> MDKINLVCGSLLHNIGKIIYRGTSERAKHSKLGGDFIKSFEQFRNTELTDCIRYHHAQEITSVKSNKEKNSLFYITYIADNISSGMDRRKDLEEGAEGFNWDKKVALGSVFNVLNEKEKGRQNYSYPFVARTRIKEEPLNFPTATQNQYTTSYYDGLITDMKTILQRLKPDKEHINSLLQMMESLWSYVPSSTDKNQLVDISLYDHSRTTAAIASAIYDYFQAENITDYQKELFDYNATEFYDKNAFLMMNFDMSGVQNFIYNISGSKALKSLRARSFYLDMLLEYISDNLLEKLELSRANILYVGGGHAYLLLANTNKTKAILSDFEHDLKTWFLDKFKIDLYVAMAYTEVSANDLMNHNGHYRDIYRRLSQKTSAKKANRYTAEEILNLNHQGTENARECRECKRSDLLIEEDDICEICDSLQKVSRDLTRENIFVIANEGVLDMPFGKKMSALSYSQADKLKKSNAEVQIYAKNISEIGQNLMTRIDMGDYTYRSDFHEMLEEVEVGINRLGVLRADVDNLGQAFINGIPDDYLSISRTATFSRAMSRFFKNYLNQLLAEKSYKINVIYAGGDDLFMIGAWQDILDFSIVLKQKFADFTQNKLSISAGIGMFREKYPVARMASLTGDLEDAAKDYKPDERAVQATKNAVTLFDATNVFSWDTLENDIFVKLDAITKNFEKLDETGKAFIYRLIDLLRGVNENQQINIARLAYTLSRMEEKIGKTFAQELYNWANADRKTLIMALEIYILKTRE;> MKIIKLYFESPVHFGEKRLSESKITFSADTLFSALMIEAVGLGKEDEFYQLASNNLVKFSDAFPFIDQYYYIPKPMFNLKLEKEDENPSKAFKKLLYVPIDSLEDYLSGGLDAYFERESFNLGKLALSEKVQQHDFKDSEPYNVGTFTFKENTGLYVLIEQTHPLLEELLENLQYSGIGGKRNSGYGKFKFEILEDSDIEDLFSAKGNRKILLSGALPKDAELEQALKNASYLLERRGGFVQSDTYATNLVKKQDLYVFKSGSTFENSFDGDIYQVGKKGNHPVYKYAKSFFLEVS;>[4x]MKLVIEGTIVLKTGMHIGGSSDFSAIGAVASPVVRDTLTRLPLIPGSSLKGKMRYLLAKELNNGILLNEPNNDQDEILRLFGSSEKDKIRRARLKFNDIKLSNLAELETFNVSSTEVKFENTINRKTAVANPRQIERVIAGSKFDFEIFYNLDDIKEVEKDFENIKQGFDLLEFDYLGGHGTRGSGRIAFENLSVITAVGNFEKINTLNEILGA;> MKKTYRVTLTALGPIFIGGGEKLKKYEYIFDKQKKVAHMIDHTKFTKYLLEKNLLDDFTSRVNSHFDLYDYLVNKKGIVFMPLVKYSVPVAQFRTEVKNRFGKPISSPPMNDLNTFVKDAFGRPYIPGSSLKGALRTAILNDLKEDTKENEVFAHLQVSDSETIDLENLKVYQKVDYSKTAKPLPLYRECLKPNTEITFTVSFDDEYLTLKKIQNALHKTYQHYYIKWLKGGKVGETLIKGVYDSHADELKKNTFALDQPSQNQGEIIYIGGGAGFVSKTLHYKSKNRDQARNDSFDILKQLFRTTYSKMRSVPDNVPVALKLAVETKTFNGRVTGKHYLEMGKARIKLEEL

The multi-subunit Type III-A CRISPR-Cas effector complex (Csm) exemplifies this principle and is in addition regulated by cellular metabolites such as divalent metals and ATP. Recognition of the foreign or cognate target RNA (CTR) triggers its single-stranded deoxyribonuclease (DNase) and cyclic oligoadenylate (cOA) synthesis activities. The same activities remain dormant in the presence of the self or non-cognate target RNA (NTR) that differs from CTR only in its 3′-protospacer flanking sequence (3′-PFS). The single-stranded DNase (ssDNase) and the cOA synthesis activities reside within the Csm1 subunit and the RNase activity resides within Csm317–19.

Interestingly, we obtained two apo structures with different stoichiometry. A second apo structure was also obtained from LlCsm without incubating with a target RNA that was refined to 2.9 Å and contains all but the Csm2 subunits (1120344151crRNA1Target0). As all Csm subunits were present immediately before making the cryoEM grids, the reason for the lack of Csm2 in the 2.9 Å apo complex is likely due to its dissociation from the complex during plunge freezing. Nearly all particles that went into the reconstruction of the apo structure contain no Csm2. Though still not clear what conditions led to the capture of the apo LlCsm in two different stoichiometries, it indicates instability of Csm2 associated with the apo complex. Thus, when Csm1 is well ordered such as in the apo state, Csm2 is loosely associated with the complex, which could lead to its disassociation. In either isolated or the CTR-bound state, Csm1 is active while in the apo or the NTR-bound state, Csm1 is inactive in cleaving non-specific DNA. In contrast, when Csm1 is bound within the apo-Csm RNP, it is immobilized in an inactivated state.(2~{R})-2-[4-[3,5-bis(chloranyl)phenyl]-3-(trifluoromethyl)phenyl]butanoic acid | C17 H13 Cl2 F3 O2 | 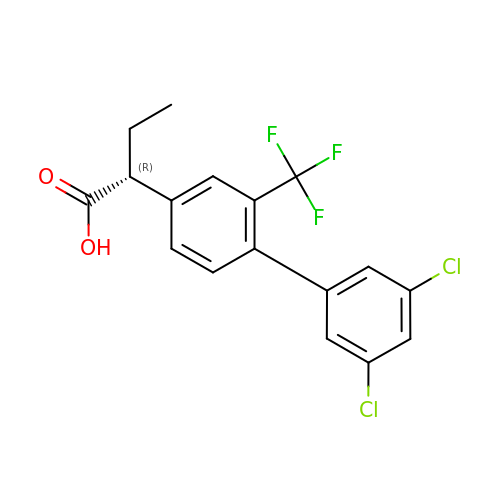MVMIGKWIRSPCJY-CYBMUJFWSA-N>[2x]MAKKTSSKGRPPGPTPLPVIGNILQIGIKDISKSLTNLSKVYGPVFTLYFGLKPIVVLHGYEAVKEALIDLGEEFSGRGIFPLAERANRGFGIVFSNGKKWKEIRRFSLMTLRNFGMGKRSIEDRVQEEARCLVEELRKTKASPCDPTFILGCAPCNVICSIIFHKRFDYKDQQFLNL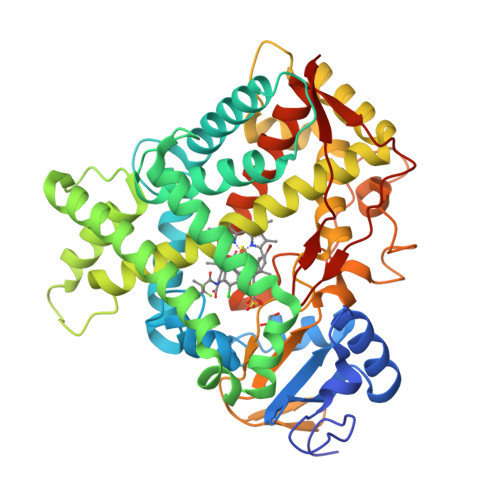MEKLNENIEILSSPWIQVYNNFPALLDYFPGTHNKLLKNVAFMKSYILEKVKEHQESMDMNNPQDFIDCFLMKMEKEKHNQPSEFTIESLENTAVDLFGAGTETTSTTLRYALLLLLKHPEVTAKVQEEIERVIGRNRSPCMQDRSHMPYTDAVVHEVQRYIDLLPTSLPHAVTCDIKFRNYLIPKGTTILISLTSVLHDNKEFPNPEMFDPHHFLDEGGNFKKSKYFMPFSAGKRICVGEALAGMELFLFLTSILQNFNLKSLVDPKNLDTTPVVNGFASVPPFYQLCFIPVHHHH> ELKIGDRVLVGGTKAGVVRFLGETDFAKGEWCGVELDEPLGKNDGAVAGTRYFQCQPKYGLFAPVHKVTKIGFPSTTPAKAKANAVR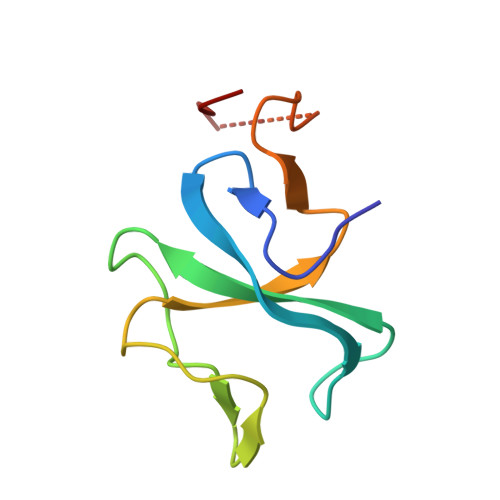RVM> GAEFHYPHVYDSQAEAMKTSAFIAGAKMILPEGIQRENNKLYEEVRIPYSEPMPLSFEEKPVYIQDLDEIGQLAFKGMKRLNRIQSIVFETAYNTNENMLICAPTGAGKTNIAMLTVLHEIRQHFQQGVIKKNEFKIVYVAPMKALAAEMTDYFSRRLEPLGIIVKELTGDMQLSKSEILRTQMLVTTPEKWDVVTRKSVGDVALSQIVRLLILDEVHLLHEDRGPVLESIVARTLRQVESTQSMIRILGLSATLPNYLDVATFLHVNPYIGLFFFDGRFRPVPLGQTFLGIKCANKMQQLNNMDEVCYENVLKQVKAGHQVMVFVHARNATVRTAMSLIERAKNCGHIPFFFPTQGHDYVLAEKQVQRSRNKQVRELFPDGFSIHHAGMLRQDRNLVENLFSNGHIKVLVCTATLAWGVNLPAHAVIIKGTQIYAAKRGSFVDLGILDVMQIFGRAGRPQFDKFGEGIIITTHDKLSHYLTLLTQRNPIESQFLESLADNLNAEIALGTVTNVEEAVKWISYTYLYVRMRANPLAYGISHKAYQIDPTLRKHREQLVIEVGRKLDKAQMIRFEERTGYFSSTDLGRTASHYYIKYNTIETFNELFDAHKTEGDIFAIVSKAEEFDQIKVREEEIEELDTLLSNFCELSTPGGVENSYGKINILLQTYISRGEMDSFSLISDSAYVAQNAARIVRALFEIALRKRWPTMTYRLLNLSKVIDKRLWGWASPLRQFSILPPHILTRLEEKKLTVDKLKDMRKDEIGHILHHVNIGLKVKQCVHQIPSVMMEASIQPITRTVLRVTLSIYADFTWNDQVHGTVGEPWWIWVEDPTN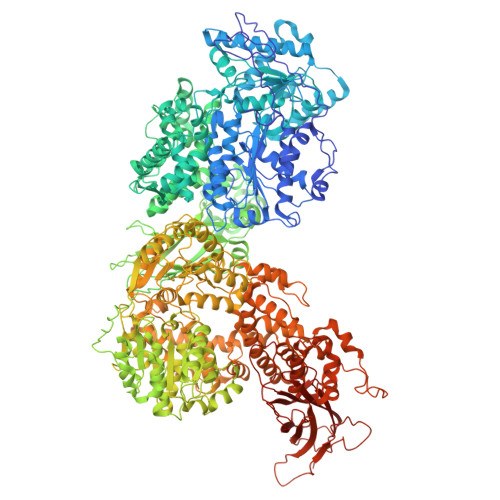DHIYHSEYFLALKKQVISKEAQLLVFTIPIFEPLPSQYYIRAVSDRWLGAEAVCIINFQHLILPERHPPHTELLDLQPLPITALGCKAYEALYNFSHFNPVQTQIFHTLYHTDCNVLLGAPTGSGKTVAAELAIFRVFNKYPTSKAVYIAPLKALVRERMDDWKVRIEEKLGKKVIELTGDVTPDMKSIAKADLIVTTPEKWDGVSRSWQNRNYVQQVTILIIDEIHLLGEERGPVLEVIVSRTNFISSHTEKPVRIVGLSTALANARDLADWLNIKQMGLFNFRPSVRPVPLEVHIQGFPGQHYCPRMASMNKPAFQAIRSHSPAKPVLIFVSSRRQTRLTALELIAFLATEEDPKQWLNMDEREMENIIATVRDSNLKLTLAFGIGMHHAGLHERDRKTVEELFVNCKVQVLIATSTLAWGVNFPAHLVIIKGTEYYDGKTRRYVDFPITDVLQMMGRAGRPQFDDQGKAVILVHDIKKDFYKKFLYEPFPVESSLLGVLSDHLNAEIAGGTITSKQDALDYITWTYFFRRLIMNPSYYNLGDVSHDSVNKFLSHLIEKSLIELELSYCIEIGEDNRSIEPLTYGRIASYYYLKHQTVKMFKDRLKPECSTEELLSILSDAEEYTDLPVRHNEDHMNSELAKCLPIESNPHSFDSPHTKAHLLLQAHLSRAMLPCPDYDTDTKTVLDQALRVCQAMLDVAANQGWLVTVLNITNLIQMVIQGRWLKDSSLLTLPNIENHHLHLFKKWKPIMKGPHARGRTSIESLPELIHACGGKDHVFSSMVESELHAAKTKQAWNFLSHLPVINVGISVKGSWDDLVEGHNELSVSTLTADKRDDNKWIKLHADQEYVLQVSLQRVHFGFHKGKPESCAVTPRFPKSKDEGWFLILGEVDKRELIALKRVGYIRNHHVASLSFYTPEIPGRYIYTLYFMSDCYLGLDQQYDIYLNVTQASLSAQVNTKVSDSLTDLALK>SFASSCTEEENNHHMGIDVIIKVTKQDQTPTNDKICQSVTEVTESEDDGVSEEVVKGDPTTYYTVVGGGLRMNFGFTKCPQIKSISESADGNTVNARLSSVSPMYGIESPAITHEEALAMINDCAVSINIKCSEEEKDSNIKTHPVLGSNISHKKV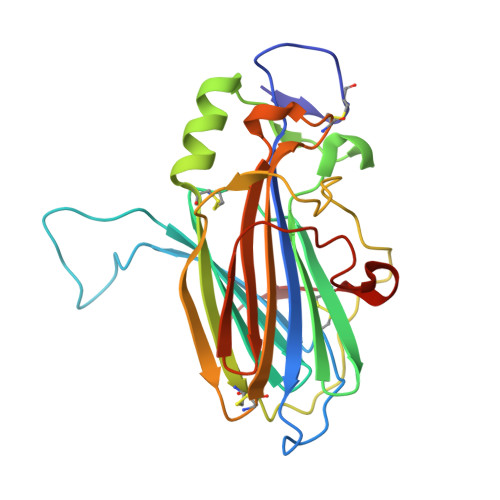RYEDIIGSTIVDIKCVKDLEFSVRIGDMCKEASELEVKDGFKYIDGSVSEGATDDTSLIDSTKLKACVGSLV[2x]> TDNTKPNRMPVAPYWTSPEKMEKKLHAVPAAKTVKFKCPSSGTPQPTLRWLKNGKEFKPDHRIGGYKVRYATWSIIMDSVVPSDKGNYTCIVENEYGSINHTYQLDVVERSPHRPILQAGLPANKTVALGSNVEFMCKVYSDPQPHIQWLKHIEVNGSKIGPDNLPYVQILKTAGVNTTDKEMEVLHLRN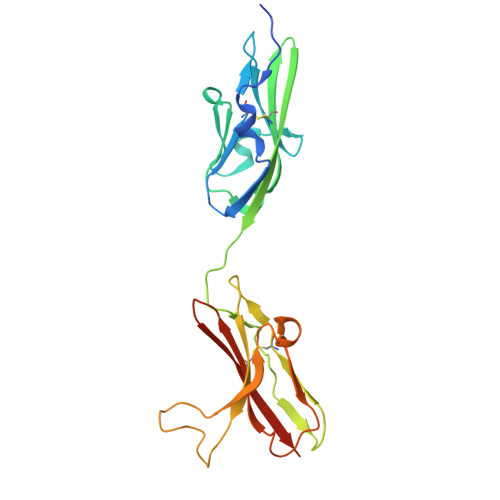VSFEDAGEYTCLAGNSIGLSHHSAWLTVLEALEER> TLSILVAHDLQRVIGFENQLPWHLPNDLKNVKKLSTGHTLVMGRKTFE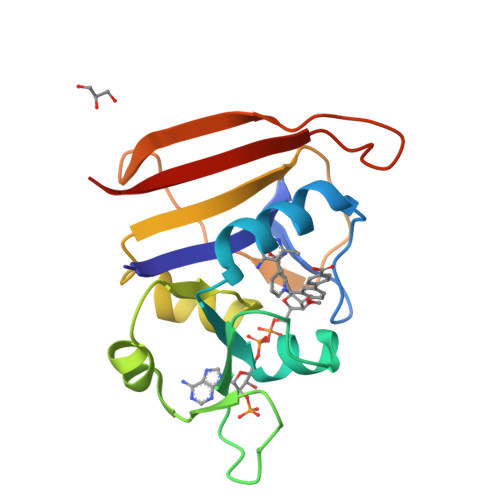SIGKPLPNRRNVVLTSDTSFNVEGVDVIHSIEDIYQLPGHVFIFGGQTLYEEMIDKVDDMYITVIEGKFRGDTFFPPYTFEDWEVASSVEGKLDEKNTIPHTFLHLIRKLEH>GPLGSRTSLIPTLGNLSNIILSILGKPVQEASAIVTNPASEMGMAFTKVMNMFRMVKDIYTEESFIYSSAIGMRTPSQRSTTRRANLAIFLAAVYGALQIGFFHLNENFLEVFAPDESNILTNQGTLYMELKTQAYISAMAQAERPKGDILNDLFPSDMAHRFLIRRNAKLDDKLTYVEKQIIEKCTARKERLANFSPQEALNEVY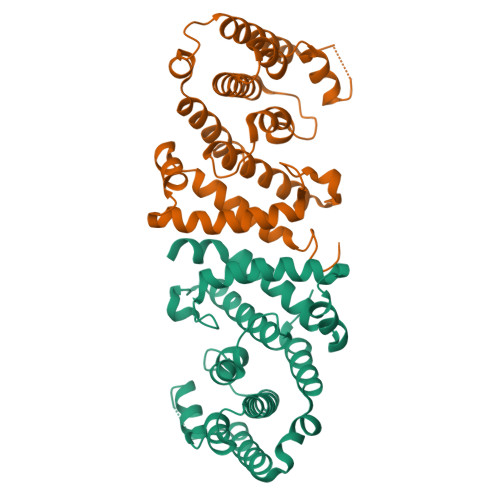PWGKFLSEIACYIHNNYSSIS[4x]>[4x]ETPTRRTGNHHPNLWDDGLIGTIQEQPYDDSHCMERAERLIGEIKDMFNESGKFCGENAFERLVMVDKVQRLAIDRHFQNEIAQALDYVYRYWSDCSRDLNSAALGLRILRLNRYPV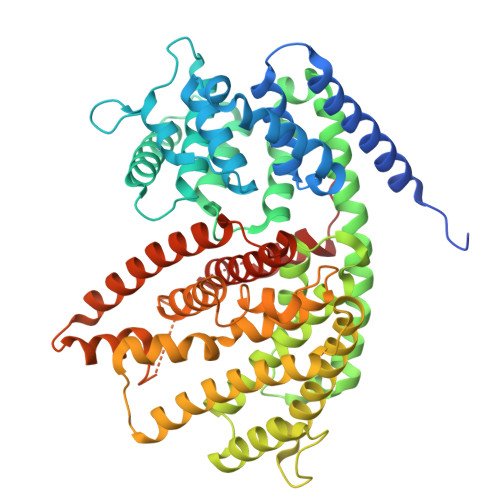SSDVLRHFKGNDGQFLCPSAQSEEEKIGSILNLYRASLIAFPEENIMDEAKAFATTYLNQVLQNNNISSHLSKEIKYNLEYGWHTNLPRVEARNYMDIYGENRSWTEMGGNMQILNLAKLDFNIMQSVHRLELESILKWWKDSNLDKVDFARHRHVEYFALACAYCIDAKYYAYRRDFAKLCALATIVDDIYDTYGTIEEIKLFNEAVKMWDSSLPNSLPENIKIAYKAFHMAVNESAEAAKKTQGRDILPYARKVWEHYLIGLTKEAEWLANGYIPSLEEYLENGAPSSGYRVTMLQPTLTLDALLPDNILLEMDYPSRFNELLCLSLRLKGDTRTFKAEANRGELVSGISCYIKDHPGSSEEEALDYLKDLLQKRLKELDQEYLKPNNVPAISKDHAYNIARSYQLLYKERDGFTNSNKDIKDLVTQILLEPIPL>[2x]GSMTHYDVVVLGAGPGGYVAAIRAAQLGLSTAIVEPKYWGGVCLNVGCIPSKALLRNAELVHIFTKDAKAFGISGEVTFDYGIAYDRSRKVAEGRVAGVHFLMKKNKITEIHGYGTFADANTLLVDLNDGGTESVTFDNAIIATGSSTRLVPGTSLSANVVTYEEQILS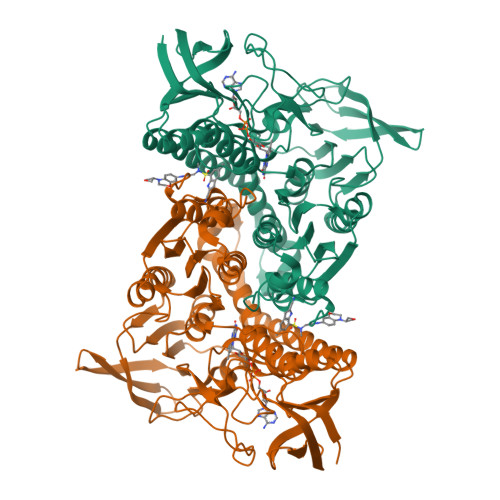RELPKSIIIAGAGAIGMEFGYVLKNYGVDVTIVEFLPRALPNEDADVSKEIEKQFKKLGVTILTATKVESIADGGSQVTVTVTKDGVAQELKAEKVLQAIGFAPNVEGYGLDKAGVALTDRKAIGVDDYMRTNVGHIYAIGDVNGLLQLAHVAEAQGVVAAETIAGAETLTLGDHRMLPRATFCQPNVASFGLTEQQARNEGYDVVVAKFPFTANAKAHGVGDPSGFVKLVADAKHGELLGGHLVGHDVAELLPELTLAQRWDLTASELARNVHTHPTMSEALQECFHGLVGHMINF>[2x]MSLDYGEFSKRFSTISGINIVPFLEGTREIDWKGLDDNVEFLLQNGIEVIVPNGNTGEFYALTIEEAKQVATRVTELVNGRATVVAGIGYSVDTAIELGKSAIDSGADCVMIHQPVHPYITDAGAVEYYRNIIEALDAPSIIYFKDAHLSDDVIKELAPLDKLVGIKYAINDIQRVTQVMRAVPKSSNVAFICGTAEKWAPFFYHAGAVGFT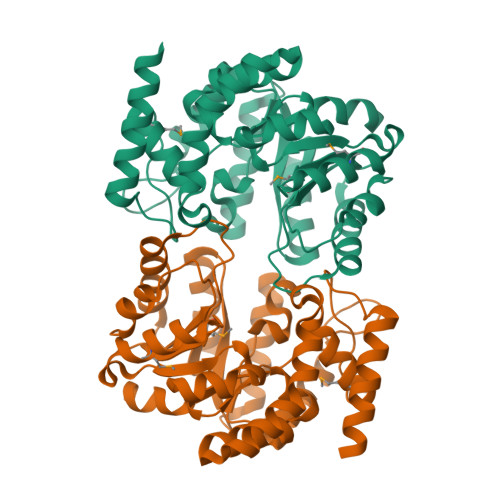SGLVNVFPQKSFALLEALEEGNQEKIWDVWEDVVPFEDLRAKHNNGNNVVIIKEAMEQLGLRAGVTREPVNPLSPNDRLELEELLKSWNTQEVREGHHHHHH> MRERTEARRRRIEEVLRRRQPDLTVLLENVHKPHNLSAI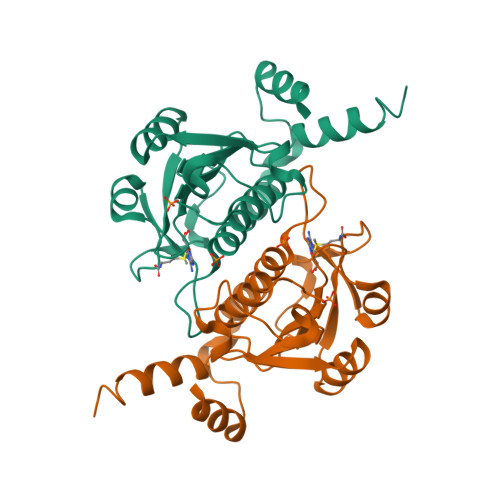LRTCDAVGVLEAHAVNPTGGVPTFNETSGGSHKWVYLRVHPDLHEAFRFLKERGFTVYATALREDARDFREVDYTKPTAVLFGAEKWGVSEEALALADGAIKIPMLGMVQSLNVSVAAAVILFEAQRQRLKAGLYDRPRLDPELYQKVLADWLRK> MTKPLDGINVLDFTHVQAGPACTQMMGFLGANVIKIERRGSGDMTRGWLQDKPNVDSLYFTMFNCNKRSIELDMKTPEGKELLEQMIKKADVMVENFGPGALDRMGFTWEYIQELNPRVILASVKGYAEGHANEHLKVYENVAQCSGGAAATTGFWDGPPTVSGAALGDSNSGMHLMIGILAALEIRHKTGRGQKVAVAMQDAVLNLVRIKLRDQQRLERTGILAEYPQAQPNFAFDRDGNPLSFDNITSVPRGGNAGGGGQPGWMLKCKGWETDADSYVYFTIAANMWPQICDMIDKPEWKDDPAYNTFEGRVDKLMDIFSFIETKFADKD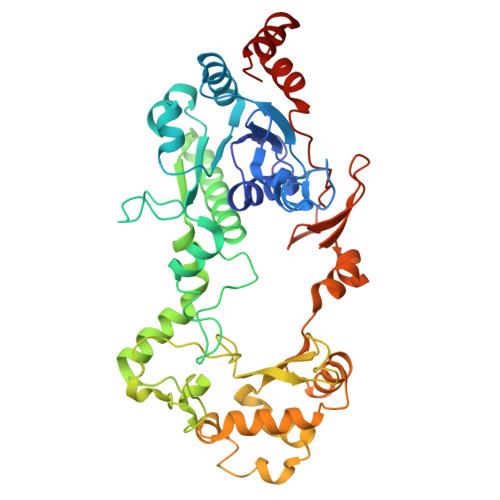KFEVTEWAAQYGIPCGPVMSMKELAHDPSLQKVGTVVEVVDEIRGNHLTVGAPFKFSGFQPEITRAPLLGEHTDEVLKELGLDDAKIKELHAKQVV>GSHMATPWSGYLDDVSAKFDTGVDNLQTQVTEALDKLAAKPSDPALLAAYQSKLSEYNLYRNAQSNTVKAFKDIDAAIIQNFR[18x]

Salmonella enterica serovar Typhimurium (S. Typhimurium), a gram-negative bacterium responsible for innumerable cases of acute gastroenteritis worldwide, utilizes two T3SSs, encoded within its pathogenicity islands 1 (SPI-1) and 2 (SPI-2), to invade cells and establish an intracellular replicative niche. The core component of this machine is the envelope-associated needle complex, which consists of a multiring base, an inner rod, and a needle filament extension that protrudes several nanometers from the bacterial surface. The entire structure is traversed by an approximately 2-nm channel that serves as a conduit for the T3SS protein substrates as they pass through the bacterial envelope. Furthermore, four residues at the end of the C-terminal α-helix, three charged (K66, D70, and R80) and one polar uncharged (Q77), form the lumen of the channel and create an electrostatic surface potential of alternating charges, which spiral upwardly about the needle, a feature that has been proposed to be important for substrate translocation.

Since we observed no differences between the structures of in vivo and in vitro polymerized needle filaments, we solved the cryo-EM structures of PrgIS49A and PrgIV67A filaments assembled in vitro from purified mutant proteins. These mutants are located within the C-terminal α-helix and resulted in specific phenotypes, such as constitutive secretion (PrgIS49A) or deficiency in the secretion of SipB (PrgIV67A). The 3D reconstruction of needle filaments assembled with PrgIV67A fell into a single class average involving more than 99% of the particles. The 3D reconstruction after 2D classification generated a map with an overall resolution of 2.9 Å. Although the helical rise is the same, PrgIV67A filaments have a smaller twist than wild type (63.27° versus 63.35°). However, no significant difference among PrgIWT, PrgIS49A, and PrgIV67A was detected in the structures of the monomers extracted from the assembled filaments, with a Cα RMSD over 77 residues of 0.152 Å between PrgIWT and PrgIS49A and 0.225 Å between PrgIWT and PrgIV67A. However, the predicted electrostatic potential of the lumens of filaments assembled with the PrgIS49A and PrgIV67A mutants showed significant differences with wild type. To clarify this issue, we fitted PrgIV67A monomer into the map of PrgIWT filaments and found that the resulting lumen electrostatic potential was essentially the same as that of the PrgIV67A filaments. These results argue that differences in helicity itself may not account for the observed differences in the electrostatic potential of the lumen surface. Rather, it suggests that slight differences in side-chain configuration may be ultimately responsible for the observed differences in the electrostatic pattern of the lumen.> ACDYTCGSNCYSSSDCSTAQAAGYKLHEDGETVGSNSYPHKYNNYEGFDFSVSSPYYEWPILSSGDVYSGGSPGADRVVFNENNQLAGVITHTGASGN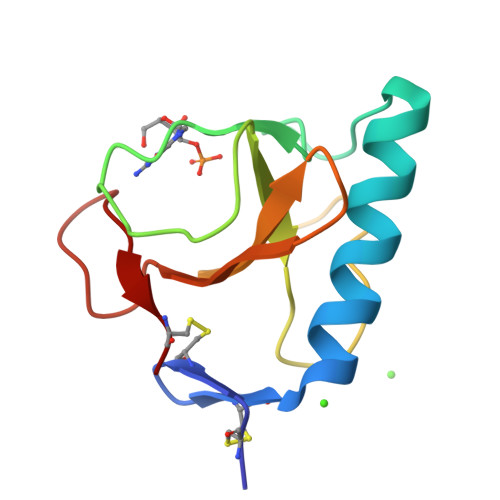NFVECT>MAHHHHHHMHEIVDKNGKKVQKNNLNDEIKIIFTALDGTLLNSENKVSEQNLESLIRAQEKGIKVVIATGRSIFSVENVIGEHVKKNRISLLPGIYMNGCVTFDEKGSRVIDRIMNNDLKMEIHEFSKQINISKYAIWFCLEKTYCFEINDCIREYMEVEALNPDVIEDNM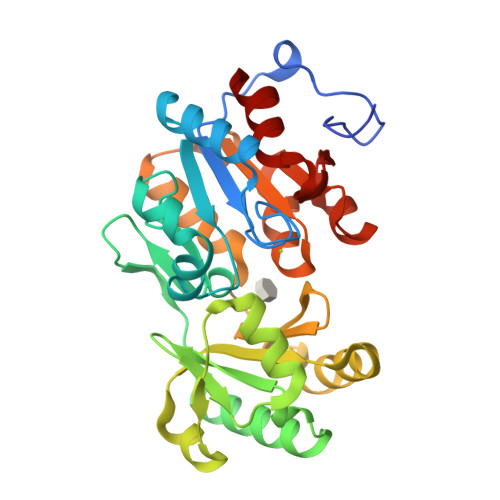LEGLTVYKVLFSLPENILENTLKLCREKFSHRINVANTFQSYVELFHQHTNKFEGVKEICKYYNISLNNALAMGDGENDIEMLSGLTHSVGVHNASEKVKNSAAYVGPSNNEHAISHVLKTFCDI[2x]> NDKLIELSNSNENWVMPGKNYDSNNYSTSTQINVDNVKQLKHAWSFSTGELHGHEGAPLVIGDVMYVHSSFPNKTFALDLNDPGHILWQHSPKQDPAARSVACCDLVNRGLAYWPGDDKTPSLIIKTQLDGHLVALNAKTGEEFWKVENGDIKVGQTLTQAPYVVHDLAIVGSSGAELGVRGHVTAYNVRTGEQAWRYYATGPDAEIGLADDFNSANPHYGQKGLGTATWEGDAWKIGGGTN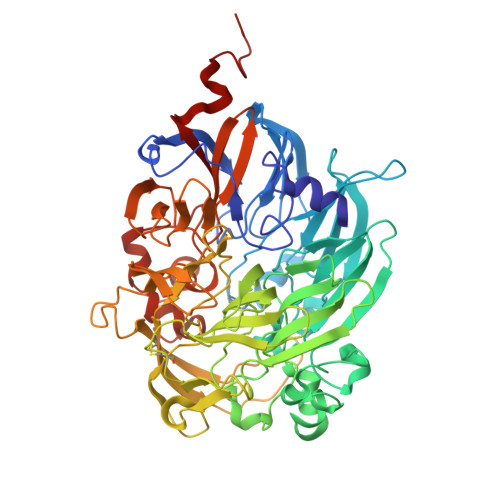WGWYAYDPAANLIYYGSGNPAPWNETMRPGDNKWTMTITARDADTGKMKFGYQKTPHDEWDFAGVNVIMLSEQTDKTGKKRKLLTHPDRNGIVYTLDRENGDLISADKLDDTVNVFKTVDLKTGLPVRDPEYGTRMDHKGTDICPSAMGYHNQGHDSYDPQKQLFFMGINHICMDWEPFMLPYRAGQFFVGATLWMYPGPKGDRQNYLGLGQIKAYNAITNEYKWQHMERFSVWGGTLATAGNLVFYGTLDGFLKARNSDTGELVWKHKLPSGVIGYPMTYEHKGVQYIAVMSGVGGWPGVGLVFDLQDPTAGLGAVGAFKNLQNYTQMGGSLEVFSLDGKNPYDDVNVGEYEKG> WGSM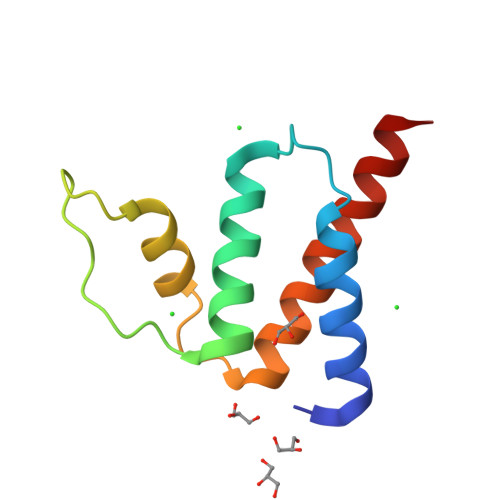GLQEDFEQYAEKAKTLPESTSNENKLILYGLYKQATVGDVNTARPGIFAQRDRAKWDAWKAVEGKSKEEAMSDYITKVKQLLEEAAAAAS> PISPIETVPVKLKPGMDGPKVKQWPLTEEKIKALVEICTEMEKEGKISKIGPENPYNTPVFAIKKKDSTKWRKLVDFRELNKRTQDFWEVQLGIPHPAGLKKKKSVTVLDVGDAYFSVPLDEDFRKYTAFTIPSINNETPGIRYQYNVLPQGWKGSPAIFQSSMTKILEPFKKQNPDIVICQYMDDLYVGSDLEIGQHRTKIEELRQHLLRWGLTTPDKKHQKEPPFLWMGYELHPDKWT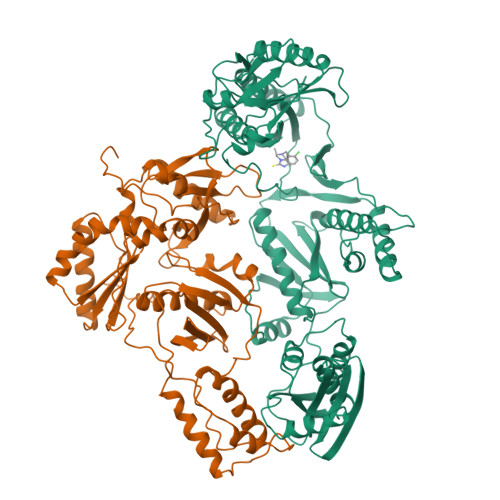VQPIVLPEKDSWTVNDIQKLVGKLNWASQIYPGIKVRQLSKLLRGTKALTEVIPLTEEAELELAENREILKEPVHGVYYDPSKDLIAEIQKQGQGQWTYQIYQEPFKNLKTGKYARMRGAHTNDVKQLTEAVQKITTESIVIWGKTPKFKLPIQKETWETWWTEYWQATWIPEWEFVNTPPLVKLWYQLEKEPIVGAETFYVDGAANRETKLGKAGYVTNKGRQKVVPLTNTTNQKTELQAIYLALQDSGLEVNIVTDSQYALGIIQAQPDKSESELVNQIIEQLIKKEKVYLAWVPAHKGIGGNEQVDKLVSAGIRK;> PISPIETVPVKLKPGMDGPKVKQWPLTEEKIKALVEICTEMEKEGKISKIGPENPYNTPVFAIKKKDSTKWRKLVDFRELNKRTQDFWEVQLGIPHPAGLKKKKSVTVLDVGDAYFSVPLDEDFRKYTAFTIPSINNETPGIRYQYNVLPQGWKGSPAIFQSSMTKILEPFKKQNPDIVICQYMDDLYVGSDLEIGQHRTKIEELRQHLLRWGLTTPDKKHQKEPPFLWMGYELHPDKWTVQPIVLPEKDSWTVNDIQKLVGKLNWASQIYPGIKVRQLSKLLRGTKALTEVIPLTEEAELELAENREILKEPVHGVYYDPSKDLIAEIQKQGQGQWTYQIYQEPFKNLKTGKYARMRGAHTNDVKQLTEAVQKITTESIVIWGKTPKFKLPIQKETWETWWTEYWQATWIPEWEFVNTPPLVKLWY>[6x]SEFTTKERKVEE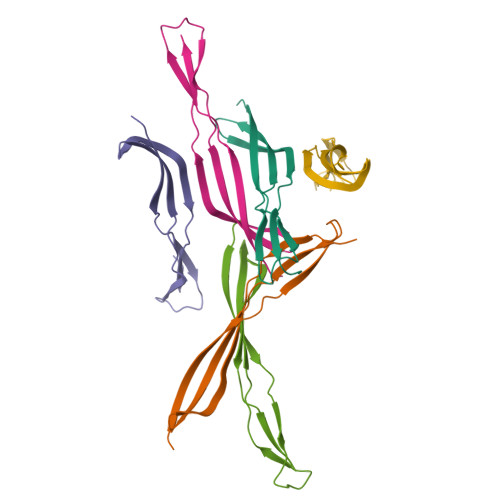ALPIKEEIRYDASLPLGKSYLLQEGKAGKKVSVYQDVIVDGKVMATNLLSETVVEGQNRILVKGSLE> MNSKSSARAAIVDTVEAVKKRKYISIEAGTLNNVVEKERKFLKQFLSGRENLRIAARVFTPCELLAPELENLGMLMYRFETDVDNPKILFVGLFFLCSNAFNVSACVRTALTTMYTNSMVDNVLSMINTCKYLEDKVSLFGVTSLVSCGSSCLLSCVMQGNVYDANKENIHGLTVLKEIFLEPDWEPRQHSTQYVYVVHVYKEVLSKLQYGIYVVLTSFQNEDLVVDILRQYFEKERFLFLNYLINSNTTLSYFGSVQRIGRCATEDIKSGFLQYRGITLPVIKLENIFVDLSEK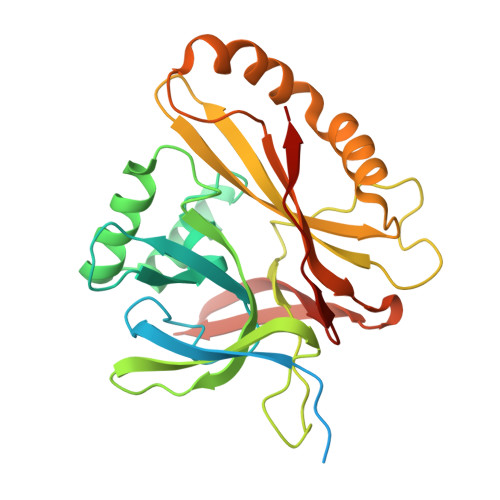KVFV> MGTTTCKQCANFFPVPKDADDYEAGKADC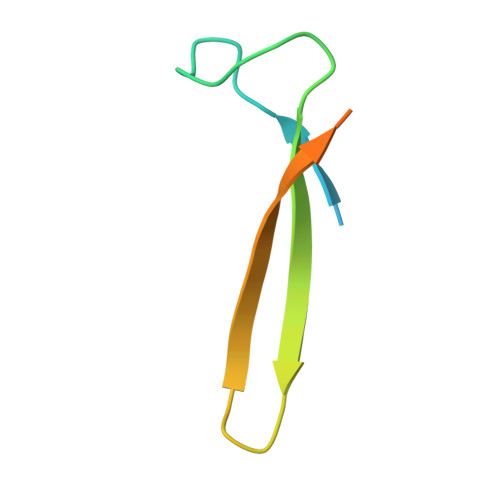VREKEDEKGKYWLSKPIFENSAQCEAFQTKR> MRGSHHHHHHGSMPFEIVFEGAKEFAQLIETASRLIDEAAFKVTEEGISMRAMDPSRVVLIDLNLPASIFSKYEVDGEETIGVNMDHLKKVLKRGKAKETLILRKGEENFLEISLQGTATRTFKLPLIDVEEI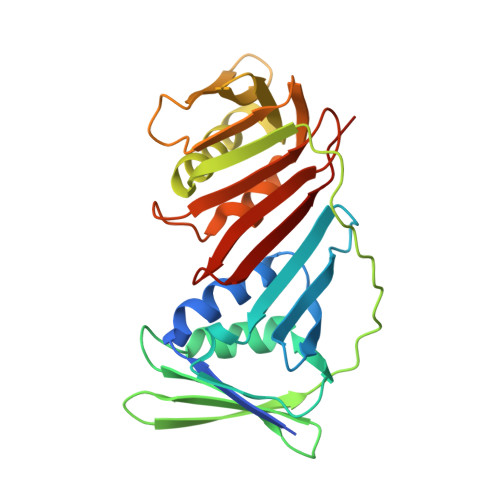EVDLPELPFTAKVVILGDVIKEAVKDASLVSDSMKFIAKENEFTMRAEGETQEVEVKLTLEDEGLLDIEVQEETKSAYGISYLSDMVKGLGKADEVTIKFGNEMPMQMEYYIRDEGRLIFLLAPRVEE> ISGMSGRKASGSSPTSPINANKVENEDAFLEEVAEEKPHVKPYFTKTILDMDVVEGSAARFDCKVEGYPDPEVMWFKDDNPVKESRHFQIDYDEEGNCSLTISEVCGDDDAKYTCKAVNSLGEATCTAELLV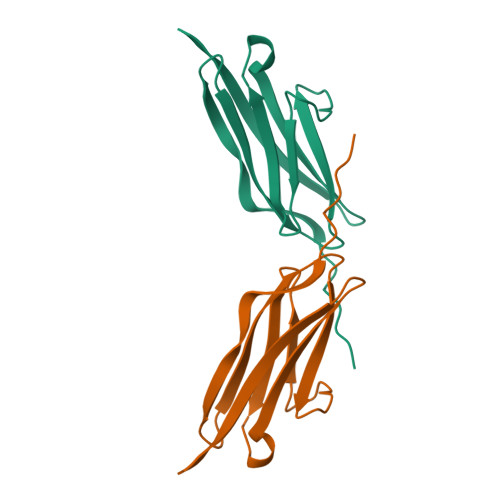ETMGKEGEGEGEGEEDEEEEEE>MTSVATKKTVQGPPTSDDIFEREYKYGAHNYHPLPVALERGKGIYLWDVEGRKYFDFLSSYSAVNQGHCHPKIVNALKSQVDKLTLTSRAFYNNVLGEYEEYITKLFNYHKVLPMNTGVEAGETACKLARKWGYTVKGIQKYKAKIVFAAGNFWGTTLS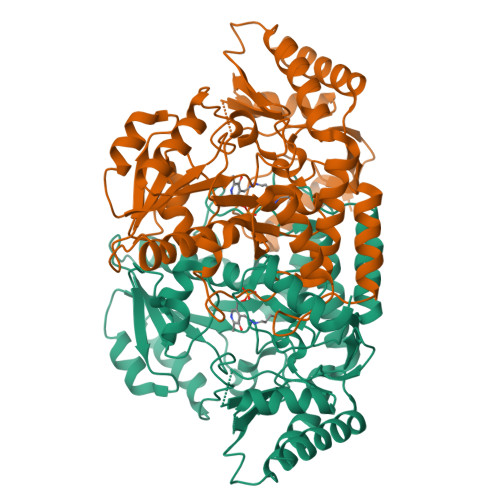AISSSTDPTSYDGFGPFMPGFDIIPYNDLPALERALQDPNVAAFMVEPIQGEAGVVVPDPGYLMGVRELCTRHQVLFIADEIQTGLARTGRWLAVDYENVRPDIVLLGKALSGGLYPVSAVLCDDDIMLTIKPGEHGSTYGGNPLGCRVAIAALEVLEEENLAENADKLGIILRNELMKLPSDVVTAVRGKGLLNAIVIKETKDWDAWKVCLRLRDNGLLAKPTHGDIIRFAPPLVIKEDELRESIEIINKTILSF[3x]>[3x]MIYGIGTDIVSLKRIIRLNKKFGQAFAGRILTPEELLEFPQAGKPVNYLAKRFAAKEAFAKAVGTGIRGAVSFRNIGIGHDALGKPEFFYGP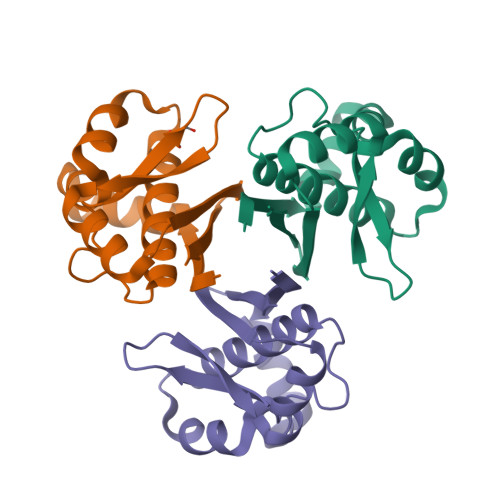ALSKWLEEQGISRVSLSMSDEEDTVLAFVVAEK>[8x]TLKGKTALVTGSTSGIGLGIAQVLARAGANIVLNGFGDPAPALAEIARHGVKAVHHPADLSDVAQIEALFALAEREFGGVDILVNNAGIQHVAPVEQFPLESWDKIIALNLSAVFHGTRLALPGMRARNWGRIINIASVHGLVGSTGKAAYVAAKHGVVGLTKVVGLETATSNVTCNAICPGWVLTPLVQKQIDDRAANGGDPLQAQHDLLAEKQPSLAFVTPEHLGEL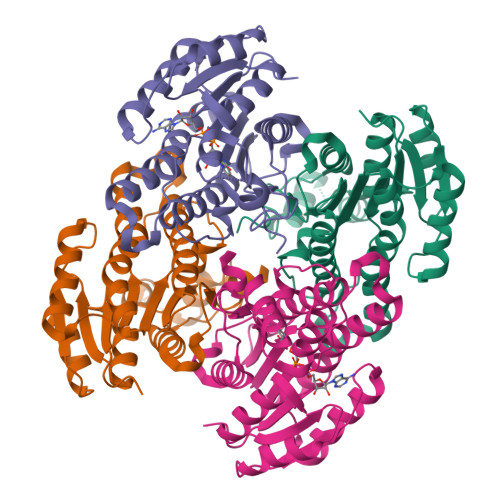VLFLCSEAGSQVRGAAWNVDGGWLAQ>[2x]MHHHHHHMNPDLRRERDSASFNPELLTHILDGSPEKTRRRREIENMILNDPDFQHEDLNFLTRSQRYEVAVRKSAIMVKKMREFGIADPDEIMWFKNFVHRGRPEPLDLHLGMFLPTLLHQATAEQQERFFMPAWNLEIIGTYAQTEMGHGTHLRGLETTATYDPETQEFILNSPTVTSIKWWPGGLGKTSNHAIVLAQLITKGKCYGLHAFIVPIREIGTHKPLPGITVGDIGPKFGYDEIDNGYLKMDNHRIPRENMLMKYAQVKPDGTYVKPLSNKLTYGTMVFVRSFLVGEAARALSKACTIAIRYSAVRHQSEIKPGEPEPQILDFQTQQYKLFPLLATAYAFQFVGAYMKETYHR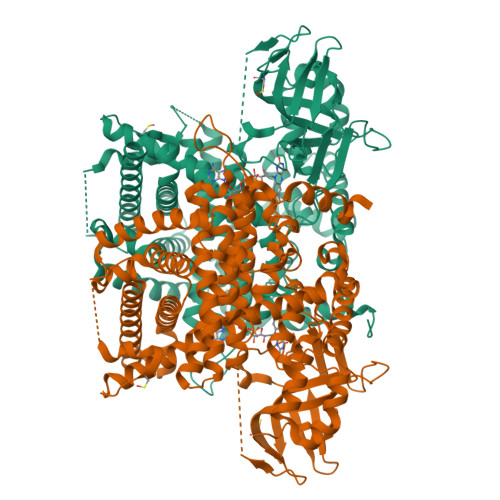INEGIGQGDLSELPELHALTAGLKAFTSWTANTGIEACRMACGGHGYSHCSGLPNIYVNFTPSCTFEGENTVMMLQTARFLMKSYDQVHSGKLVCGMVSYLNDLPSQRIQPQQVAVWPTMVDINSPESLTEAYKLRAARLVEIAAKNLQKEVIHRKSKEVAWNLTSVDLVRASEAHCHYVVVKLFSEKLLKIQDKAIQAVLRSLCLLYSLYGISQNAGDFLQGSIMTEPQITQVNQRVKELLTLIRSDAVALVDAFDFQDVTLGSVLGRYDGNVYENLFEWAKNSPLNKAEVHESYKHLKSLQSKL>[2x]MSHLLLFVTLLGAFGLGYLQGGPVLGLFLAGLGLLLGRGLRPAR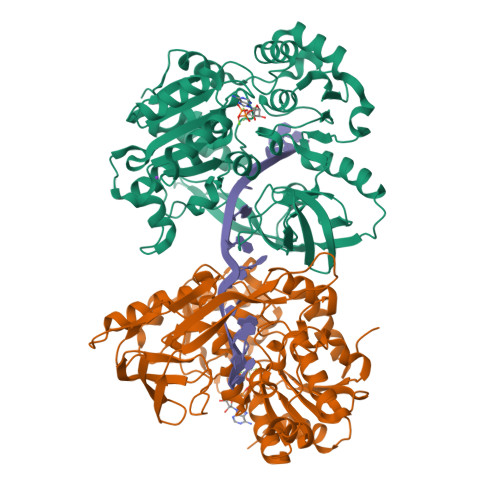PSQVEEPPSPKADPEEVEETPEGLSSEQQRAFLAVTQTPHPAHLITGPAGTGKTTLLYALQEFYKGRAVTLAPTGTAALQARGQTVHSFFRFPARLLRYRHPEDIRPPGPHSPLRKAIEQMEVLILDEVGMVRVDLLEAMDWALRKTRKRLEEPFGGVKVLLLGDTRQLEPVVPGGEEALYIARTWGGPFFFQAHVWEEVALRVHRLWESQRQREDPLFAELLKRLRQGDPQALETLNRAAVRPDGGEEPGTLILTPRRKEADALNLKRLEALPGKPLEYQAQVKGEFAETDFPTEAALTLKKGAQVILLRNDPLGEYFNGDLGWVEDLEAEALAVRLKRNGRRVVIRPFVWEKIVYTYDSEREEIKPQVVGTFRQVPVRLAWALTVHKAQGLTLDKVHLELGRGLFAHGQLYVALTRVRRLQDLSLSRPIAPTELLWRPEVEVFETRIQEGIWQKSHGWPSL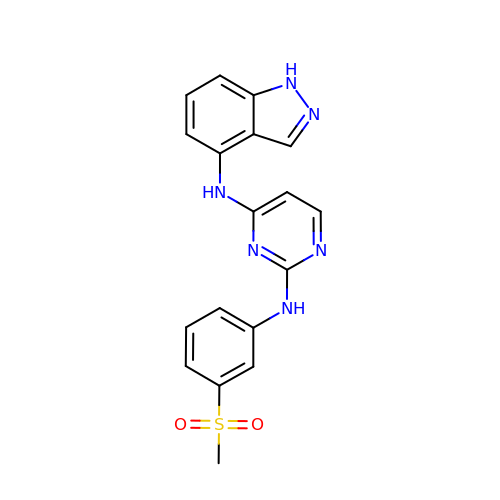N^4^-1H-INDAZOL-4-YL-N^2^-[3-(METHYLSULFONYL)PHENYL]PYRIMIDINE-2,4-DIAMINE | C18 H16 N6 O2 S | FIWCLCRWDUELGO-UHFFFAOYSA-N> MRTTKKIVSAVLAACMLASTAVVSSFAATADDSSAVSSDYARDNSYTKAAEDIDAQYAYSGNDLGVTYTKDATTFKVWSPTATGVKLNIFTKGSDDEQGASKVASYTLEKMLVDGEWNGVWTITLVGEWKDYYYTYSVTTTDTTHIGSDATKTYETQDVYSTATGVNGKRSMIVDLDETDPEGWSNDSHVLLDKSTKSSVWELHIKDFSYDKASGVSDANRGKYLAFTENGTTLNGEGKVSTCIDYLKELGVTTVQLNPFYDFQSVNEAGDDSQFNWGYDPVNYNVPEGSYSSNPYDGKVRIKECKEMIKALHDAGISVVMDVVYNHTYSTDSCFQYTVPNYYYRMKTTGAFSDGSGCGNEGATERAMYRQYVIDSLKYWVNEYHVDGFRFALMGLMDVETMNMAREALDQIDPRITMWGEGWAGGDSYHPTNTCSGTKFYPATQANASRLSDRIAIFNDGIRDGIKGSAMDISDVGFIQGSKSSAKGVSYGVRANSSGTYKWKAQAPSQCVTYDACHDNATLYDQIIASTGLADYGERNSEAVKMNRLASAIIYTSQGISFTLAGEEMARSKDGDTNSYKSAANLNMIKWQNVVDYADVVSYYKGMMQIKSAFSPLTAMDNSYADKYTFTKKVSASTNQISF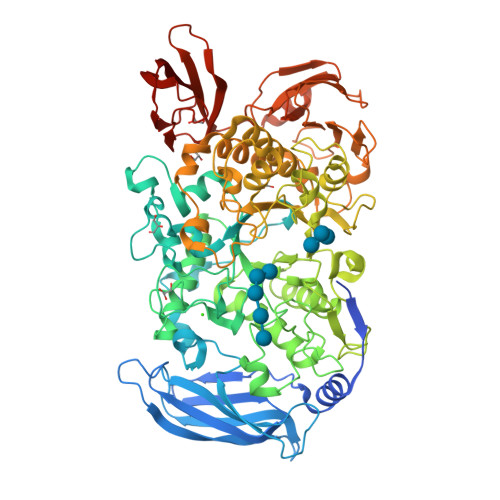TIQNDVEGEWNKMAVIYNNATTAADVTLSDTSVTDWVVIANGETAGLDSLGEVTGSTFTVPARSAIVAVDKAGYESAGIHSSKGKVKVNYVYEATGEKLEDSVILQGSVGSGYVTVPSAVIPDTYIVSRIGGNAEGKYTSDMQEVTYYYTDYIP> PISPIETVPVKLKPGMDGPKVKQWPLTEEKIKALVEICTEMEKEG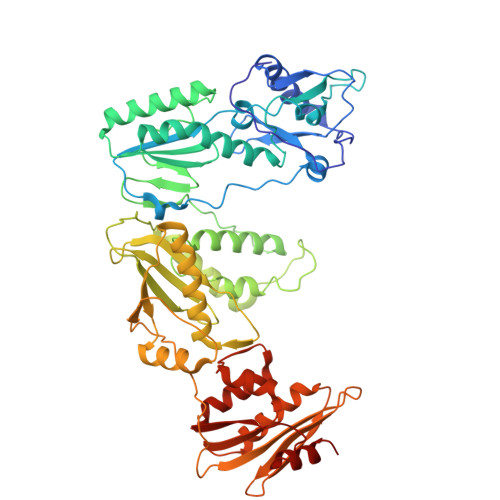KISKIGPENPYNTPVFAIKKKDSTKWRKLVDFRELNKRTQDFWEVQLGIPHPAGLKKKKSVTVLDVGDAYFSVPLDEDFRKYTAFTIPSINNETPGIRYQYNVLPQGWKGSPAIFQSSMTKILEPFKKQNPDIVIYQYMDDLYVGSDLEIGQHRTKIEELRQHLLRWGLTTPDKKHQKEPPFLWMGYELHPDKWTVQPIVLPEKDSWTVNDIQKLVGKLNWASQIYPGIKVRQLSKLLRGTKALTEVIPLTEEAELELAENREILKEPVHGVYYDPSKDLIAEIQKQGQGQWTYQIYQEPFKNLKTGKYARMRGAHTNDVKQLTEAVQKITTESIVIWGKTPKFKLPIQKETWETWWTEYWQATWIPEWEFVNTPPLVKLWYQLEKEPIVGAETFYVDGAANRETKLGKAGYVTNKGRQKVVPLTNTTNQKTELQAIYLALQDSGLEVNIVTNSQYALGIIQAQPDKSESELVNQIIEQLIKKEKVYLAWVPAHKGIGGNEQVDKLVSAG Cytochromes c′ occur in methanotrophic, denitrifying and photosynthetic bacteria and have proposed roles in protection against nitrosative stress, NO trafficking during denitrification or pathogen defence. All cytochromes c′ have a 4 α-helix bundle structure containing a heme centre with a solvent exposed proximal His ligand and a buried hydrophobic distal pocket with a non-coordinated residue (Leu or Phe, rarely Met or Tyr) in a position to exert steric influence on the binding of diatomic gases. Unusually, cytochromes c′ are able to utilize both heme faces (distal and proximal) as a means of discriminating NO from other diatomic gases. In order to understand the factors controlling distal versus proximal NO coordination, we have examined NO binding to AXCP variants in which the occluding distal residue Leu16 is replaced with residues that are smaller (Ala, Val), of comparable size (Ile) or larger (Phe).

The Fe–N–O angles for these are very similar (136° and 139°) and only one conformer of Ile16 is present. Ile16 undergoes a modest shift in position (∼0.9 Å) upon binding of NO while maintaining a similar rotamer. In this structure, the heme 7-propionate is not flipped to the proximal pocket (as observed in the 6c–CO complex of wt AXCP) but does have an altered conformation. For example, the L16V and L16I structures exhibit multiple Fe–N–O conformers, whereas there is no evidence for multiple sets of heme–NO RR bands in solution. 6on values for L16V (1.52 ± 0.03 × 106 M–1 s–1) and L16I (1.79 ± 0.15 × 106 M–1 s–1) are midway between those of L16A and wt AXCP, consistent with intermediate residue sizes and steric constraints.

> QFAKPEDAVKYRQSAITLMASHFGRMTPVVKGQAPYDAAQIKANVEVLKTLSALPWAAFGPGTEGGDARPEIWSDAASFKQKQQAFQDNIVKLSAAADAGDLDKLRAAFGDVGASCKACHDAYRKK Phot2 is a high-intensity blue-light photoreceptor mediating phototropism in higher plants. The protein comprises two successive light–oxygen–voltage (LOV) domains (LOV1 and LOV2) separated by the α-helix A′α, and a kinase domain separated from LOV2 by the α-helix Jα [Fig. 1(a)]. In particular, Jα unfolds upon blue-light irradiation, triggering kinase activity. TR-SOX was used to probe the build up of the light state in the photocycle of the LOV2 domain of Phot2 (phototropin-2) from Arabidopsis thaliana (AtPhot2LOV2) with a time resolution of 63 ms.

The dark state of AtPhot2LOV2 absorbs light maximally at λ = 447 nm via its flavin mononucleotide (FMN) chromophore. To determine the structure of the dark state of AtPhot2LOV2, representative of the time series before t = 0 ms, we carried out the same diffraction experiment, but without illumination, on a series of 32 crystals. The first 500 images of 15 data sets could be successfully integrated and were subjected to clustering with ccCluster which retained 5 sub-wedges using a CCthreshold of 0.43 and resulted in a complete highly redundant data set at 2.2 Å resolution. Most residues were modelled in a single conformation A, while ten were modelled with alternate conformations A and B, including Cys426 which forms a covalent bond with the FMN in the light state. The hydro­philic side of the FMN isoalloxazine ring is stabilized by two hydrogen bonds to Asn458 and one key hydrogen bond to Gln489 [Fig. 4(a)].

> MEKNFVISDPRLPDNPIIFASDSFLELTEYSREEILGRNCRFLQGPETDQATVQKIRDAIRDQREITVQLINYTKSGKKFWNLFHLQPMRDQKGELQYFIGVQLDGEFIPNPLLGLDSTRTGHHHHHH1-methyl-6-oxidanylidene-~{N}-(2-pyrrolidin-1-ylethyl)pyridine-3-carboxamide | C13 H19 N3 O2 | 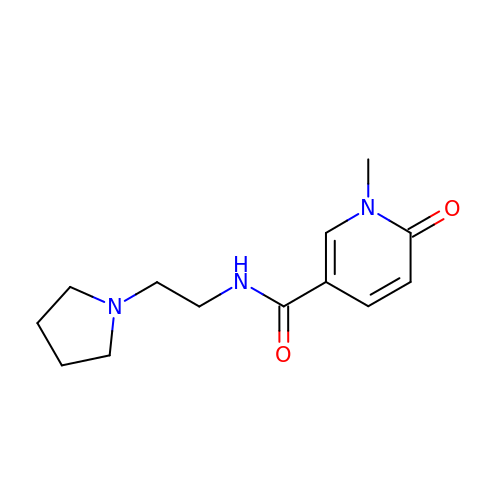BHVHUAARAHRDNS-UHFFFAOYSA-N>[5x]MDKYNNYSNVIKNKSSISPLLAAAAKIEPEITVLSSASKSNRSQYSQSLADTLLGLGYRSIFDIAKVSRQRFIKRHDESLLGNGAVIFDKAVSMANQVLQKYRKNRLEKSNSPLVPQTSSSTDASSESQTNKLPEYNQLFPEPWDNFCRPGAIEALDSPASYLLDLYKFIQSVELDGSNQARKLETRRADIPKLSLDNDALYKEVTALSIVNDVLSGSAREYIDQSGQADKAVNQILGDTHFPFTLPYSLPTQQINKGLGASNIELGTVIQRVDPQFSWNTTQEKYNQVLLAYTQLSSEQIALLSLPDVFTQNFLTQTELSAGYLSASTTEILAEKDLSRHGYIVKAADNIKGPTQLVEHSDASYDVIELTCTNQAKETITVKLRGENIITYQRTKARMVPFDNSSPFSRQLKLTFVAEDNPSLGNLDKGPYFANMDIYAAEWVRENVSSETMVSRPFLTMTYRIAIAKAGASLEELQPEADAFFINNFGLSAEDSSQLVKLVAFGDQTGSKAEEIESLLSCGENLPIVSPNVIFANPIFGSYFNDEPFPAPYHFGGVYINAHQRNAMTIIRAEGGREIQSLSNFRLERLNRFIRLQRWLDLPSHQLDLLLTSVMQADADNSQQEITEPVLKSLGLFRHLNLQYKITPEIFSSWLYQLTPFAVSGEIAFFDRIFNREQLFDQPFILDGGSFTYLDAKGSDAKSVKQLCAGLNISAVTFQFIAPLVQSALGLEAGTLVRSFEVVSSLYRLVSIPQTFGLSTEDGLILMNILTDEMGYLAKQPAFDDKQTQDKDFLSIILKMEALSAWLTKNNLTPASLALLLGVTRLAVVPTNNMVTFFKGIANGLSENVCLTTDDFQRQELEGADWWTLLSTNQVIDDMGLVLDIHPVWGKSDEEMLMEKIQSIGVSNDNNTLSIIVQILIQAKNAQENLLSQTISAEYGVERSVVPLQLRWLGSNVYSVLNQVLNNTPTDISSIVPKLSELTYSLLIYTQLINSLKLNKEFIFLRLTQPNWLGLTQPKLSTQLSLPEIYLITCYQDWVVNANKNEDSIHEYLEFANIKKTEAEKTLVDNSEKCAELLAEILAWDAGEILKAASLLGLNPPQATNVFEIDWIRRLQTLSEKTMISTEYLWQMGDLTENSEFSLKEGVGEAVMAALKAQGDSDNV;>[5x]MSNSIEAKLQEDLRDALVDYYLGQIVPNSKDFTNLRSTIKNVDDLYDHLLLDTQVSAKVITSRLSLVTQSVQQYINRIALNLEPGLSINQQEATDWEEFANRYGYWAANQQLRMFPEIYVDPTLRLTKTEFFFQLESALNQGKLTDDVAQKAVLGYLNNFEEVSNLEIIAGYQDGIDIENDKTYFVARTRMQPYRYFWRSLDASQRNANSQELYPTAWSEWKAISVPLENVANGIVRPIMMDNRLYISWFEVAEEKETDSDGNIIVSGRYRTKIRLAHLGFDGVWSSGTTLREEVLADQMEEMIAVVDRMEDEPRLALVAFKEMSESWDVVFSYICDSMLIESSNLPTTTHPPKPGDGDKGLSDLDDYGANLVWFYLHETANGGKAEYKQLILYPVIINRDWPIELDKTHQGDFGTVDDFTLNSNYTGDELSLYLQSSSTYKYDFSKSKNIIYGIWKEDANNNRCWLNYKLLTPEDYEPQINATLVMCDKGDVNIITGFSLPNGGVDAGGKIKVTLRVGKKLRDKFQIKQFSQTQYLQFPEASSADVWYIGKQIRLNTLFAKELIGKASRSLDLVLSWETQNSRLEEAILGGAAELIDLDGANGIYFWELFFHMPFMVSWRFNVEQRYEDANRWVKYLFNPFECEDEPALLLGKPPYWNSRPLVDEPFKGYSLTQPSDPDAIAASDPIHYRKAVFNFLTKNIIDQGDMEYRKLQPSARTLARLSYSTASSLLGRRPDVQLTSFWQPLTLEDASYKTDSEIRAIEMQSQPLTFEPVVHDQTMSAVDNDIFMYPMNNELRGLWDRIENRIYNLRHNLTLDGKEINMDLYDSSISPRGLMKQRYQRVVTARNASKMNFKVPNYRFEPMLNRSKSGVETLIQFGSTLLSLLERKDSLSFDAYQMIQSGDLYRFSIDLQQQDIDINKASLEALQVSKQSAQDRYDHFKELYDENISSTEQKVIELQSQAANSLLMAQGMRTAAAALDVIPNIYGLAVGGSHWGAPLNAAAEIIMIKYQADSSKSESLSVSESYRRRRQEWELQYKQAEWEVNSVEQQINLQNMQIKAANKRLEQVEAQQQQAMALLDYFSERFTNESLYTWLISQLSSLYLQAYDAVLSLCLSAEASLLYELNLGEQSFVGGGGWNDLYQGLMAGETLKLALMRMERVYVEQNSRRQEITKTISLKALLGESWPAELNKLKQKTPINFNLEEQIFVEDYQELYQRRIKSVSVSLPMLVGPYEDVCAQLTQTSSSYSTRADLKTVENMLTKRTFADTPHLVRSIQPNQQISLSTGVNDSGLFMLNFDDERFLPFEGSGVDSSWRLQFTNLKQNLDSLNDVILHVKYTAAIGSSTFSQGVRKILANINNDE;>[5x]MVNKYTYTSSKAMSDISDVIGEPLAAWDSQVGGRVFNVIFDGKVYTNTYWVERWQVPGIGSSDGNPHNAWKFVRAATADEI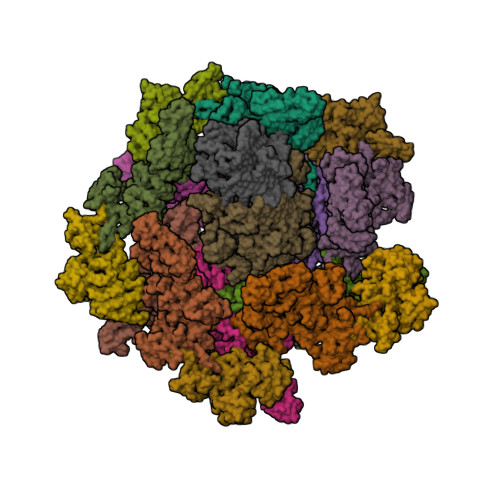NKIGNPTTADVKPTENIPSPILVEDKYTEETYSRPDVNFKEDGSQGNLSYTATRVCAPMYNHYVGDKTKPKLSAYITDWCQYDARLDGGGSKEEERGRGFDLATLMQNPATYDRLIFSFLGICGDIGNKSKKVQEVWDGWNAQAPSLGLPQIGKGHIVPLDPYGDLGTARNVGLPPESADTSIESGTFLPYYQQNRAAGLLGGLRELQKKAHAMGHKLDLAFSIGGWSLSSYFSALAENPDERRVFVASVVDFFVRFPMFSCVDIDWEYPGGGGDEGNISSDKDGENYVLLIKELRSALDSRFGYSNRKEISIACSGVKAKLKKSNIDQLVANGLDNIYLMSYDFFGTIWADYIGHHTNLYSPKDPGEQELFDLSAEAAIDYLHNELGIPMEKIHLGYANYGRSAVGGDLTTRQYTKNGPALGTMENGAPEFFDIVKNYMDAEHSLSMGKNGFVLMTDTNADADFLFSEAKGHFISLDTPRTVKQKGEYAAKNKLGGVFSWSGDQDCGLLANAAREGLGYVADSNQETIDMGPLYNPGKEIYLKSISEIKSK;> MQNSQEMAITTLSLPKGGGAINGMGESVGQAGPDGMVTFSIPLPFSAGRGVAPALSLSYSSGAGNGPFGMGWQCSAMSISRRTQKGVPQYNEDDEFLSPSGEVMAIALNDSGFEDVRTANRLQGIPLPFSYKVTRYQPRLIQDFIKIEYWQPVKQTDGTPFWIIYSPDGQTHILGKNSHSRVANAENPSQIASWLLEETVTPTGEHIYYQYSGENQVNCTDAEIALHPQDSAQRYLARIDYGNISPQASLFVLDEELPNLTQWLFHLVFDYGERDISINKIPTFEGGTTGWLARPDMFSRYDFGIEIRNRRLCHQVLGFHRLEALNDRDVTDEIPVLVNRLTLDYDLNNSVSTLVAVRQVAYETDGSPITQPPLEFDYQRFDTGSIPGWQEMPQLEAFNGYQPYQMIDLYGEGTPGILYQETPGAWWYKSPQRQIGGDSNAVTYGAMKALPKIPRLQEGATLMDINGDGRLDWVITSAGVRGFHSIHSTGEWTHFTPLNTLPTEYFHPKAQLADLVGAGLSDLVLIGPKSVRLYANQQGNWAPAQDVTQAENVSLPVIGIDSRQLVAFADMLGSGQQHLVEITADSVKCWPNMGHGRFGQPLTLEGFSQPQTSFNPDRVFLADIDGSGTNDIIYAHSECLEIYLNESGNRFSKPISLLLPDGVNFDNTCQLQAADIQGLGIASLVMTVPHMSPTHWRCDLALNKPWLLNVMNNNRGAETCLFYRSSAQFWLDEKQLVEAAGQQPECHLPFPMHLHWRSEIFDEITGNRLTQEQEYAHGSWDGQEREFRGFGRLIQRDTDGFAQGTVDIPTHPSRTVSWFATGIPEIDTTLSAEFWRGDDQAFSPFSPRFTRWENDSEAGSDVAFIPSEHDAFWLNRAMKGQLLRSELYGDDGTPEAEIPYSVTEMRHQVRALPTTDATVPSAWCSTIETRSYQYQRVAADPQCSQQVVIKADRYGSPLLSVAINYPRRKKPEKSPYPDDLPETLFDSSYDTQQQQLHLTKQQQNYFHLTNDDNWLLGLPKEQRNDGYQYDQERAPANGFTLETLIASNSLIGSNQPFTYLGQSRVAYQGGVDEQPSLQALVAYGETAILDEKTLQAFVGVLDSKTRDELLFSAGYQLAPRLFRVESEPDVWVARQGYSEFGDYSQFWRPLSQRSTLLTGKTTLKWDKHYCVVIETQDAAQLVTQARYDYRFLTPYSLTDANDNQHYVVLNPFGEVIASRFWGTEAGKDAGYSTPQAKPFVVPATIEAALALSPGIPVAHCAIFEPESWMQKLTQHDVSERMADNGTLWNALLQARFVTEDGYVCALGRRRWMARHGLSVLMLTLLAEIPRTPPHSLTITTDRYDSDDQQQLRQRILFSDGFGRLLQSAQRVEAGESWQRSEDSSLVVNVSGTPALVVTDNRWAVSGRTEYDGKGQGIRVYQPYFLDDWRYLSDDSARTDLFADTHIYDPLGREYQVITAKGYRRERQYTPWFVVNQDENDTAANLAI;> MDIQLFSKTPSVTVFDNRGLSVRDIAYRRHPDTPKVTEECITYHQFDFRGFLAQSLDPRLNHKEVTNFSYLTDLNGNIIYTQSVDAGNTLVLNDTEGRSVIAMTNISRGENGKDDLSLAVTRTFQYENAPLPGRPLSVTEQVNGENARITEHFVYAGNTPQEKNLNLAGQCVSYYDAAGLIQTDSVSLTGKPLSVSRKLLKNLDDTNILADWQGNDTSAWNSLLATEIYTTVTRTDAAGAVLTTIDAVGNQQRVAFDIAGQLSASWLTLKGGQEQVIIKVLTYSAAGQKLREEGGNGVVTTYTYEAETQRLIGIKTERPNGHAAGAKVLQDLRYEYDPVGNVLSITNDAEETRFWRNQKVVPENAYRYDSLYQLVSASGREVAGAGQQGSDLPSPLVPLPSDSSVYTNYTRTYTYDSAGNLMRIRHSAPATNNNYTLNITVSERSNRGVMSSLTENPADVDALFTASGSQKCLQQGQSLIWTPRGELRTVLLVARGETADDSESYRYDGSSQRILKISSQQTNHSARVQRALYLPGLEWRTMTGGVAEAENLQVICIGEAGRAQVRVLHWESGKPDGIINDQIRWSYDNLTCSSGLEVDGDGLVISMEEYYPYGGTAVWAARSHIETAYKTVRYSGKERDATGLYYYGFRYYQPWAGRWLSADPAGTVDGLNLYRMVRNNPLRLTDPDGMAPLDWLDLDTTNASRDIVKAIYQLNQIDGPHRGVRDTYQRMTESTGMILQETLNNEAVLKGIKQKDKEKKSRGMKFTNSKLKTYAAHAGVLNTLQPDPVYKDGFLNLPGSLGNKNTFPGVELIEDKVKPSLSQYHPDKLGKSQRWKPESSLGYYRVADTEAFITGIRSQYKSSGTDLHAVVEGRIRDHLLANNNVLPKMAGIAGLHAEVQALNYIISNPDIEGGNAERLNGSYIFTQRLVGDVNQDFPACYNCSGIISGLENVMTGRVNNDVRLKRRKSF> MLRRLAGCVAFRKNVVRPFMNSTALLSSPPAAVSAPVIPKSGNEGKDYSVASGSVDTPVLDQLVGYYVNIQSRKMYYKDFLRIEHQAVRWAFADIRKNSEALAHGLLQTGLRPGQRVLAIQPCNCETFVLQLACAKIGALLAVVPHHNISADKLRFYLNEFQPHHLIAREWIVVPEVKQGVLVERNMHFWDMIYNVIPELGLSYPGQRFQWVHSQEFFFLKKVVI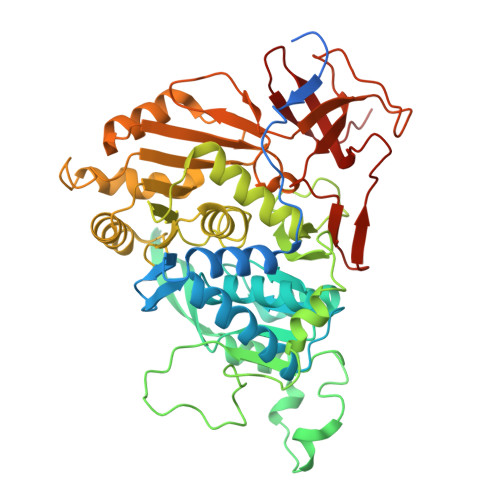TDHNMNLLGVTPMRKMLVWGPFSYYEQRLRRLSALLHPDDPILALEDPHPALEDKLHITYSHRNCINAGFLFGNLMGLKAESRFGVMPNHHVDPVGAIVAPYAALTTGAVLVHIHSDMFTDDHAINGIEKLCVEEVVGMLGKKSDFDLLLRHAGNFDADQYEHLKWVVLFEDASEPTVGDEYLQKLAKELGLEDVFVFRGPLESAYMVMWRSLKRARWEMVPHVEAKVVGDRGTADARILAANTRGNLKLKGPHISAGYYNNAGLLTELVDERGFCSTSREAVMDERGQLTLHGTQLY>CCCGGG[6x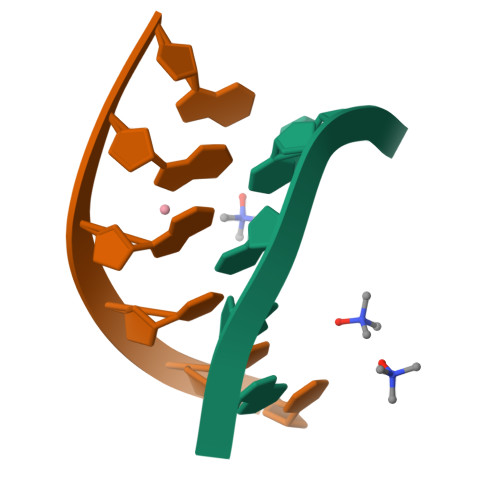]> TGGVQTVTLIPGDGIGPEISAAVMKIFDAAKAPIQWEERNVTAIQGPGGKWMIPSEAKESMDKNKMGLKGPLKTPIAAGHPSMNLLLRKTFDLYANVRPCVSIEGYKTPYTDVNIVTIRENTEGEYSGIEHVIVDGVVQSIKLITEGASKRIAEFAFEYARNNHRSNVTAVHKANIMRMSDGLFLQKCREVAESCKDIKFNEMYLDTVCLNMVQDPSQFDVLVMPNLYGDILSDLCAGLIGGLGVTPSGNIGANGVAIFESVHGTAPDIAGKDMANPTALLLSAVMMLRHMGLFDHAARIEAACFATIKDGKSLTKDLGGNAKCSDFTEEICRRVKDLD;> FSEQTIPPSAKYGGRHTVTMIPGDGIGPELMLHVKSVFRHACVPVDFEEVHVSSNADEEDIRNAIMAIRRNRVALKGNIETNHNLPPSHKSRNNILRTSLDLYANVIHCKSLPGVVTRHKDIDILIVRENTEGEYSSLEHESVAGVVESLAIITKAKSLRIAEYAFKLAQESGRKKVTAVHKANIMKLGDGLFLQCCREVAARYPQITFENMIVDNTTMQLVSRPQQFDVMVMPNLYGNIVNNVCAGLVGGPGLVAGANYGHVYAVFETATRNTGKSIANKNIANPTATLLASCMMLDHLKLHSYATSIRKAVLASMDNENMHTPDIGGQGTTSEAIQDVIRHIRV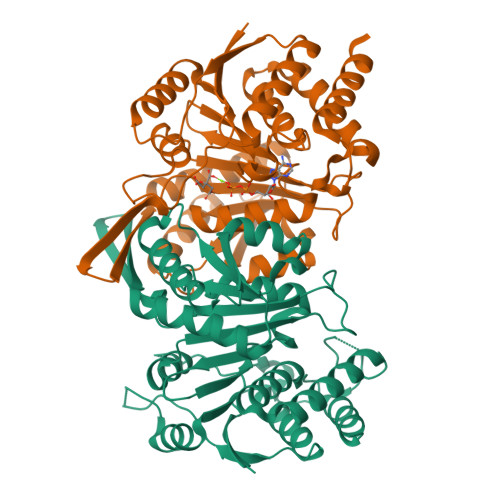INGRAVEA Inorganic pyrophosphatase (PPase) catalyses the hydrolysis reaction of inorganic pyrophosphate (PPi) to two inorganic phosphates (Pi) and plays an essential role for living organisms. We previously reported the expression and purification of family II PPase from the psychrophilic Shewanella sp. AS-11 (Sh-PPase) isolated from shellfish living in the Southern Ocean (Antarctic Ocean). Sh-PPase activated by Mn2+ ions (Mn-Sh-PPase) displayed the highest activity at 5 °C, which is characteristic of cold-adapted enzymes. X-ray crystallography and EPR spectroscopy were used to investigate a cold-adapted family II Sh-PPase from a psychrophilic bacterium that lives in the Southern Ocean.

The crystal structure of Mn-Sh-PPase in the absence of substrate was determined at 2.2 Å resolution. The M1 and M2 sites showed similar coordination spheres to other family II PPases. The M1 site in Mn-Sh-PPase was coordinated with one nitrogen of histidine, two oxygens of aspartates (D12 and D72), and a bridged water. Additionally, the M1 site was bound with an extra water molecule. Coordination geometry of the M2 site in Mn-Sh-PPase was also similar with that of Bs-PPase and Sg-PPase with 5-coordinated bipyramidal geometry. However, the distances of a bridged water in the Sh-PPase from M1 and M2 (3.0 and 2.4 Å, respectively) were considerably longer compared with crystal structures of other di-Mn enzymes. In addition to the Mn-O distance, the Mn-Mn distance of Sh-PPase was also longer than arginase and catalase. A unique structural feature of Mn-Sh-PPase found in the present X-ray analysis is the longer distance between bridged water and two Mn atoms compared with that in other family II PPases. Our observations reveal that the di-Mn centre of Mn-Sh-PPase in both single crystal and solution forms has longer distance with bridged water. This suggests that the active site of Mn-Sh-PPase has an intrinsically ‘loose’ structure.

>MGSMYVVGHKIPDSDSICGAIALAYLKNQIGEPAIAARLGELSPETAFILEKFGFEAPEYKTSYAGEEVYIVDHSEITQAPDDIAQATIVGIVDHHKLGDLTTSTPLECWIRPVGCSNTVIKMMYDFYQVKIPANIAGIMMCAILSDTVIFKSPTCTTADIRCVEALAEIAGVEDFKEVGMDMFKVKSAVEGTPARDLVMRDFKDFNMNGNLVGIGQLEVIDLAVFDDIKADLEADIAKLKVEGNRHSVLLLLTDIMKEGSEMLVVSDSADLTERAYGKPTVDGRVWLDGVLSRKKQVVPALQDAFQKV[4x]> MGHHHHHHGQQDVHGPFQGQRQNEFDLMFVKEIFKNHNSNVVLSPFSVKILLTLIYEASDTSFGNAVSNTKRELSSVIQNDNIDHTRSYYKQLLESAQQ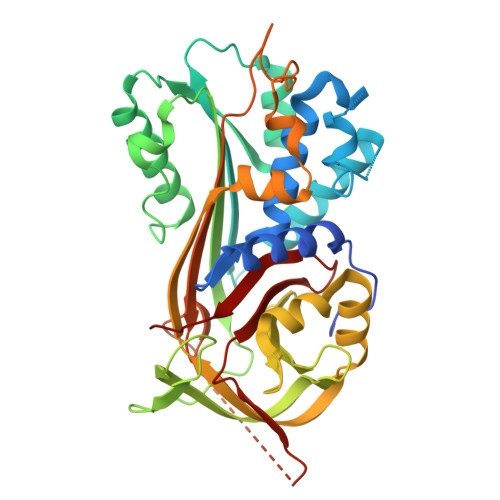DNKDYDLNIATNFFVDDFIEVINKYQQIANTHYHAMLEKVSYSNPTQTAATINNWVSEHTNGRLREIVTPDSLEGAVITLVNVIYFKGLWTYPFPEVANNVKPFYGTRGKPTNAQYMEQNGQFYYDNSADLGAQILRLPYRGNKLAMYFILPNPDNTVNQVLDRINSASLHQALWYMEENEVNVTLPKFKFDFSEQLNEPLQQVGIREIFSQNASLPLLARGRGARDEVRVSRIFQKAGITINELGWEAYAATEIQLVNKFGGDGVQIFNANRPFIFFIEDETLGTMLFAGKIENPVF>[2x]MHHHHHHMDYLPERDVYESLCRGEGVKLTPRRQKRLFCRYHHGNRAPQLLIAPFKEEDEWDSPHIVRYYDVMSDEEIERIKEIAKPKLARATVRDPKTGVLTVASYRVSKSSWLEEDDDPVVARVNRRMQHITGLTVKTAELLQVANYGVGGQYEPHFDFSRNDERDTFKHLGTGNRVATFLNYMSDVEAGGATVFPDLGAAIWPKKGTAVFWYNLLRSGEGDYRTRHAACPVLVGCKWVSNKWFHERGQEFL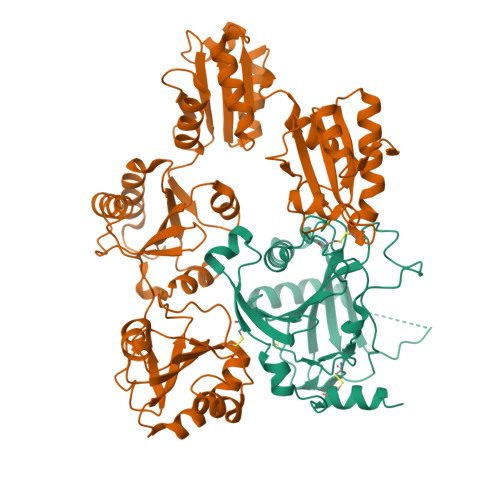RPCGSTEVD;>MDAPEEEDHVLVLRKSNFAEALAAHKYLLVEFYAPWCGHCKALAPEYAKAAGKLKAEGSEIRLAKVDATEESDLAQQYGVRGYPTIKFFRNGDTASPKEYTAGREADDIVNWLKKRTGPAATTLPDGAAAESLVESSEVAVIGFFKDVESDSAKQFLQAAEAIDDIPFGITSNSDVFSKYQLDKDGVVLFKKFDEGRNNFEGEVTKENLLDFIKHNQLPLVIEFTEQTAPKIFGGEIKTHILLFLPKSVSDYDGKLSNFKTAAESFKGKILFIFIDSDHTDNQRILEFFGLKKEECPAVRLITLEEEMTKYKPESEELTAERITEFCHRFLEGKIKPHLMSQELPEDWDKQPVKVLVGKNFEDVAFDEKKNVFVEFYAPWCGHCKQLAPIWDKLGETYKDHENIVIAKMDSTANEVEAVKVHSFPTLKFFPASADRTVIDYNGERTLDGFKKFLESGGQDGAGDDDDLEDLEEAEEPDMEEDDDQKAVKDEL[2x]> ISNYKYLE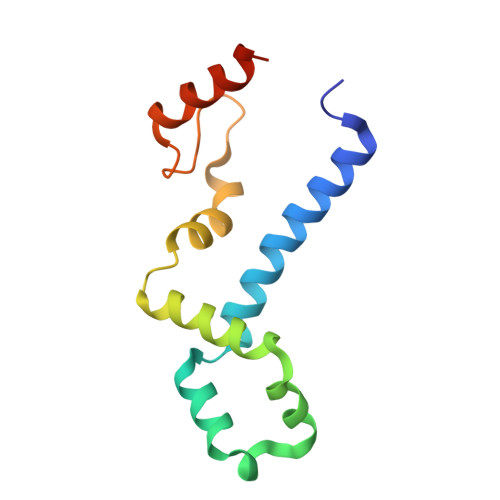VIQLEHAVTKLVESYNKIIELSPNLVAYNEAVNNQDRVPVQILPSLSRYQLKLAAELKTLHDLKKDAILTEITDYENEFDTEQKQPILQEISKADMEKLEKLEQVKREKRE>[2x]GFSFELTEQQKEFQATARKFAREEIIPVAAEYDRTGEYPVPLLKRAWELGLMNTHIPESFGGLGLGIIDSCLITEELAYGCTGVQTAIEANTLGQVPLIIGGNYQQQKKYLGRMT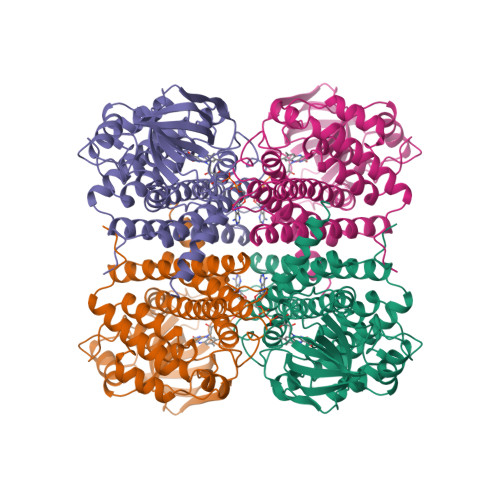EEPLMCAYCVTEPGAGSDVAGIKTKAEKKGDEYIINGQKMWITNGGKANWYFLLARSDPDPKAPASKAFTGFIVEADTPGVQIGRKEINMGQRCSDTRGIVFEDVRVPKENVLTGEGAGFKIAMGTFDKTRPPVAAGAVGLAQRALDEATKYALERKTFGKLLAEHQGISFLLADMAMKVELARLSYQRAAWEIDSGRRNTYYASIAKAYAADIANQLATDAVQVFGGNGFNTEYPVEKLMRDAKIYQIYEGTAQIQRIIIAREHIGRYK>[4x]ALSKVVIRRLPPTLTKEQLQEHLQPMPEHDYFEFFSNDTSLYPHMYARAYINFKNQEDIILFR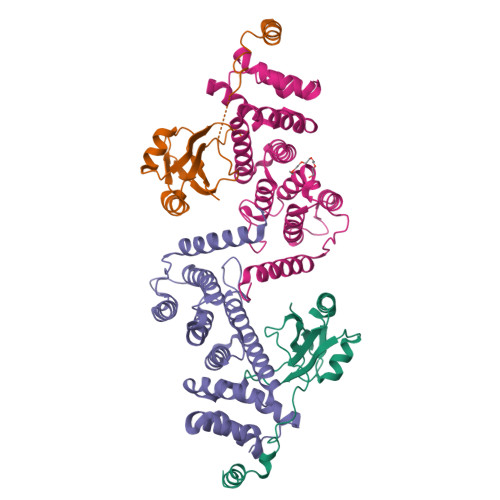DRFDGYVFLDNKGQEYPAIVEFAPFQKAAKKKTKKRDTKVGTIDDDPEYRKFLESYATD;>[4x]KRPPLQEYVRKLLYKDLSKVTTEKVLRQMRKLPWQDQEVKDYVICCMINIWNVKYNSIHCVANLLAGLVLYQEDVGIHVVDGVLEDIRLGMEVNQPKFNQRRISSAKFLGELYNYRMVESAVIFRTLYSFTSFGVNPDGSPSSLDPPEHLFRIRLVCTILDTCGQYFDRGSSKRKLDCFLVYFQRYVWWKKSLEVWTKDHPFPIDIDYMISDTLELLRPKIKLCNSLEESIRQVQDLEREFLIKLGLVNDK>[2x]SMDKLKKIDQTIHAFYCEKAVISEKLNEAVLYSINAGGKRIRPILFLEVIEALQIPLTESHFKAAAALEMIHTGSLIHDDLPAM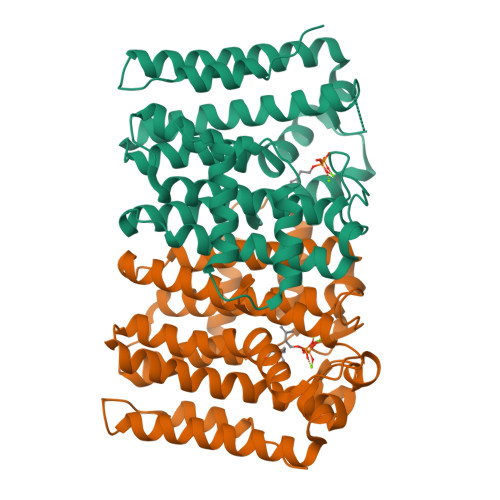DNDDYRRGQLTNHKKFDEATAILAGDSLFLDAFGMLAETDFPTDVTVDLVRSLSSASGTFGMVGGQMLDMAAEGKKLNLKNLQLIHRHKTGQLLAYPFWAAARVAQLDENLLATFLEIGMIIGLAFQVRDDILDITANFEEIGKTPKKDVMAEKMTYPHLLGLNESYQILDESLDQAEAILRKLSDEIAFAPQKILSLIERLRLDA> GTRVLIVGGSLVGLSTAVFLAHHDVPVTLVERHPGTSIHPRAVGYYPRTAELLATVGVEAPAKAAASG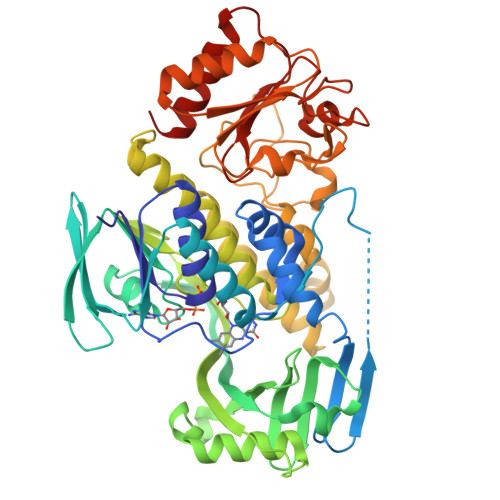FEKHRTRAGVESLAGEVLFSKEELEGGDELADLTPSSLLLLPQDRLEPILRARAEELGAELRFGAELRSFTQDADGVSAVVRDADGGESVVRADYLVAADGPRSTVREALGIGREGRGVLSRHVSIAFGADFAAVLGERRYSVVHVQNDRVTGILVHDDTLTEGTLIVGYDPEKGEGLDDFTDARCAELVSAAIGSDDVAVTIRSRFPWDMAELVADAFVSDRVLVAGDAAHQIPPTGGYGANTGIADAFNLSWKLAHVLAGTAGRALLDTYDEERRPVGLYTARQGSLQLAVRSRTATEEQREAAHDAMRVTMGQAYPSGAFVADAGADPLPLTSDPRTLRGEPGTRAPYVVLERDGAPLSTLDLFGDGFVLLVGADGGSWAEAAGEAAAGLGVGIAFHRVAPDAGEGRPVDVHGRWAEAYGVGAAGAVLVRPDGIVAWRSRDGMPGGAGGRALTAALRTVLAR> MRRRTVISFGYVRVAASAVGVIGMGANHRHHYQQQQRPITTRGQFNPVHDFTYAMERGVRARDEKTFEKLITNPGPLRIAYSPDYLDWLYRCYKAKGKYMDARAAAEKKFNGNIISGGAVTTSSGEMIHPLPGAPPPGMFLRPPNSFRRLSGEMKRKHAQETLDEVSKAQGMLDLFERQPQFPAIHIDRCTRFHLVELFKEMVLERSLEAVAIWDKALLYRAILSERKASYPASFRYIFKAVEDTVFAHSSVNCPSLEAYYYFLYLVKKYYIDNAVEAHVVLRCHREPNATDLLFSNPPPKDEVDVRNAIEALQSAEATSHAASSATSGTAKHDDPAATDEKHTRGDNDQKDSANANAKHPCQFAPPSSYPPIEALWRCEENVPLLEILLFGEFNLIVSENPFVKFPTAHAFLTRPYSTESSKGPIDGASLANVIAEKRGHLLPSFPMNVASAIDGRAQELRRLQQKHHRDDTVSFQTLLRSTHVDDNPSTFSSYSDWSYFNPRAVRAEERDRLT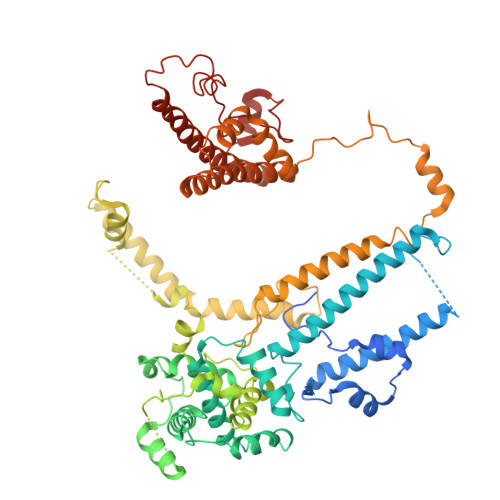RKGIDALKEYDSATEDIYRRSFEDAQASNFQRVTEAWNTFPPYLPTLPHFVSIIKKDSHISFLLHVGLPERCSSAEAAAKHKEFERRIYQLARALYHTALEFHKETVRRVNRQKVNVAASLLDNFFEQEWVAMLRESESLENSLEQGAWPDKKTDMARRLGRYIPFARRSLDENGFPTDARADDYARWMEAPARMKGAA>[2x]APKNELVQKFQVYYLGNVPVAKPVGVDVINGAL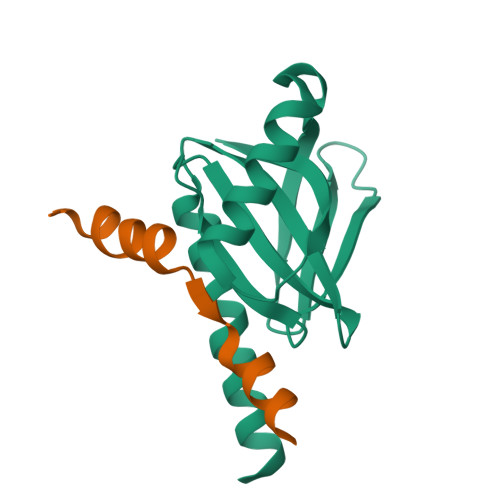ESVLSSSSREQWTPSHVSVAPATLTILHQQTEAVLGECRVRFLSFLAVGRDVHTFAFIMAAGPASFCCHMFWCEPNAASLSEAVQAACMLRYQKCLDARSQHHHHHH;>GAMDAAVAPEERHLSKMQQNGYENPTYKFFEQMQN[2x]>[2x]GINDLDISPIDPQTGGSFDQQGVFVKGYAMLGVTGQKGIDGSPDLDGQDEGESGFYRTTFNCNELPTDECLWAWQKNQDIPQLTSISWSPSSQRTEWVYVRLGYDITQYNFFLDQTEGMTDAETLRQRAEIRFLRALHYWYFLDLFGKAPFKEHFSNDLPVEKKGTELYTYIQNELNEIEADMYEPRQAPFGRADKAANWLLRARLYLNAGVYTGQTDYAKAEEYASKVIGSAYKLCTNYSELFMADNDENENAMQEIILPIRQDGVKTRNYGGSTYLVCGTRVAGMPRMGTTNGWSCIFARAAMVQKFFSNLEDVPMLPADVEIPTKGLDTDEQIDAFDAEHGIRTEDMIKAAGDDRALLYSGVGGGRRKIQ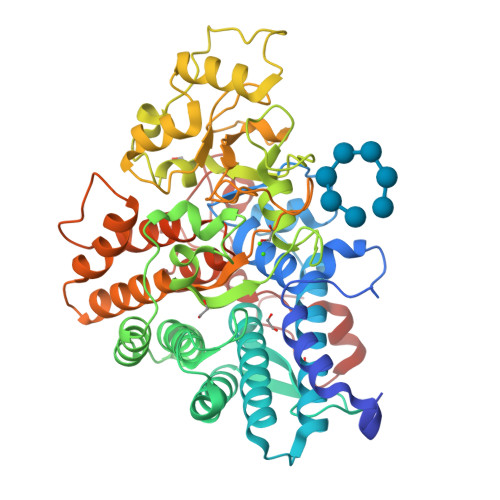TDAISGFTDGLSIVKWQNYRSDGKPVSHATYPDTDIPLFRLAEAYLTRAEAIFRQGGDATGDINELRKRANCTRKVQTVTEQELIDEWAREFYLEGRRRSDLVRFGMFTTNKYLWDWKGGAMNGTSVASYYNKYPIPVSDINNNRNMSQNEGYK Rspo (R-spondin, also roof plate-specific spondin) proteins are evolutionarily conserved from fish to humans and have well-documented roles in a broad range of developmental and physiological processes resulting from enhancement of canonical and non-canonical Wnt signalling. ZNRF3/RNF43 specifically targets these Wnt receptors for ubiquitination and turnover, hence reducing Wnt signalling responses. Direct extracellular interaction with Rspo proteins inhibits ZNRF3/RNF43 activity. Here we report a molecular level analysis of the ZNRF3/RNF43 ectodomain structure and its interactions with Rspo proteins.

The crystal structures of the ZNRF3ecto–Rspo2Fu1–Fu2 and RNF43ecto–Rspo2Fu1–Fu2 complexes revealed a 1:1 interaction between Fu1 of the Rspo2Fu1–Fu2 and a single ZNRF3ecto or RNF43ecto chain. Neither the Rspo2Fu1–Fu2 nor the ZNRF3ecto dimer show major conformational changes on complex formation. The first, extensive, area of interaction involves hydrophobic interactions interspersed with hydrophilic (complementarily charged) patches contributed by the first two β-hairpins of the Rspo Fu1 and the region immediately carboxy-terminal to the β3 strand of ZNRF3ecto. The Met-finger at the tip of the second β-hairpin of Fu1 nestles into a pocket formed between the β3 strand and the αC–β7 loop of the ZNRF3ecto, which is lined with hydrophobic residues (I95, I191, V192, A198). The αC–β7 loop is a flexible region in the unliganded ZNRF3ecto crystal structures and moulds to interface the RspoFu1–Fu2 M68 in the complex. Overall, the ZNRF3ecto dimer structure appears less flexible in the complex structures compared with the unliganded structures. The acidic region of the β3–β4 loop (immediately adjacent to C104 of the disulphide bridge) becomes more ordered in the ligand-bound ZNRF3ecto structures, probably as a result of electrostatic interactions with a positively charged patch on Rspo Fu1. For all ZNRF3ecto–Rspo2Fu1–Fu2 complex structures we determined (from five different combinations of species and crystal forms), the dimer found in most of the unliganded ZNRF3ecto crystal structures reoccurs. The overall assembly thus comprises a 2:2 complex of ZNRF3ecto–Rspo2Fu1–Fu2. The 2:2 complex resembles a crab with the ZNRF3ecto dimer forming the body from which the two Rspo2Fu1–Fu2 ligands diverge, without interacting with each other, as the pincers.

>[2x]ETGESLAKETAFVEVVLFESSPNGDYKTHTTELQGRFSRAGATISAEGEIVQMHPLGLCNNNDEEDLYEYGWVGVVKLEQPEMDPKPCLTVLGKAKRAVQRGATAVIFDVSDNPDAVEQLNQGLEDPLKRPVVYMKGMDAIKLMNIVNKQKGARARIQHRPPRQPTEYFDGTHHHHHHHHHH;>[2x]ETGGTNPICKGCLSCSKDNGCLRCQPKLFFYLRREGMRQYGECLQSCPPGYYGVRGPDMNRCSRCRIENCDSCFSRDFCIKCKSGFYSHKGQCFEECPEGFAPLDDTMVCVDGTKHHHHHH The central mechanism for electron transfer across the membrane involves the Mtr complex, a porin-cytochrome complex that consists of periplasmic decaheme MtrA, a large transmembrane pore MtrB, and the decaheme cytochrome MtrC on the surface of the cell. MtrC is extended approximately 80 Å above the lipid bilayer of the cell membrane, providing a surface for extracellular electron transfer to environmental substrates. MtrC is composed of four domains: an N-terminal β-barrel domain (domain I) is followed by a pentaheme domain (domain II), a second β-barrel domain (domain III), and a C-terminal pentaheme domain (domain IV). Domain III contains a conserved CX8C motif, which forms a disulfide bond between the two cysteines.

MtrCC453Asol was crystallized, and a structural model was determined to a resolution of 1.9 Å. The overall structure was almost identical to the wild-type structure with a root mean square displacement (RMSD) of 0.297 Å. The area around Cys453 was largely conserved, although Fo-Fc maps revealed a negative patch of density where the disulfide was formed between Cys453 and Cys444 in MtrCsol. This confirmed that Cys453 was replaced with alanine and the disulfide was missing, but there were no other significant changes in the environment near residue 453. In addition, there was no electron density consistent with the covalent attachment of anything to Cys444. These data show that the Cys453 substitution caused little perturbation of MtrC beyond the removal of the disulfide within the second β-barrel domain of MtrC. For MtrCsol, the presence of FMN doubled the amount of peroxide formed, while for MtrCC453Asol, there was a greater than 5-fold increase in the amount of peroxide formed, with a peroxide/electron efficiency of ~1%. The fluorescence spectrum of the isolated complexes revealed copurification of FMN with MtrCC453Asol but not MtrCsol, consistent with the reduced forms of FMN and MtrC heme facilitating an increase in the affinity of FMN for MtrCC453Asol. Normalized spatial discrepancy (NSD) values between the MtrC model and the molecular envelopes were 1.17 (MtrCC453Asol) and 1.28 (MtrCsol), suggesting that, while neither solution model fitted the structure perfectly, MtrCC453Asol in solution more closely resembles the crystal structure than MtrCsol. In our MtrCC453A isoform, the formation of the disulfide bond is prevented, trapping MtrCC453A into a state that favors FMN reduction under aerobic conditions, leading to increased production of peroxide and cell damage.

> MMNAQKSKIALLLAASAVTMALTGCGGSDGNNGNDGSDGGEPAGSIQTLNLDITKVSYENGAPMVTVFATNEADMPVIGLANLEIKKALQLIPEGATGPGNSANWQGLGSSKSYVDNKNGSYTFKFDAFDSNKVFNAQLTQRFNVVSAAGKLADGTTVPVAEMVEDFDGQGNAPQYTKNIVSHEVCASCHVEGEKIYHQATEVETCISCHTQEFADGRGKPHVAFSHLIHNVHNANKAWGKDNKIPTVAQNIVQDNCQVCHVESDMLTEAKNWSRIPTMEVCSSCHVDIDFAAGKGHSQQLDNSNCIACHNSDWTAELHTAKTTATKNLINQYGIETTSTINTETKAATISVQVVDANGTAVDLKTILPKVQRLEIITNVGPNNATLGYSGKDSIFAIKNGALDPKATINDAGKLVYTTTKDLKLGQNGADSDTAFSFVGWSMCSSEGKFVDAADPAFDGVDVTKYTGMKADLAFATLSGKAPSTRHVDSVNMTACANCHTAEFEIHKGKQHAGFVMTEQLSHTQDANGKAIVGLDACVTCHTPDGTYSFANRGALELKLHKKHVEDAYGLIGGNCASCHSDFNLESFKKKGALNTAAAADKTGLYSTPITATCTTCHTVGSQYMVHTKETLESFGAVVDGTKDDATSAAQSETCFYCHTPTVADHTKVKM>[5x]GAMDIAAQAKLVYHLNKYYNEKCQARKAAIAKTIREVCKVVSDVLKEVEVQEPRFISSLNEMDNRYEGLEVISPTEFEVVLYLNQMGVFNFVDDGSLPGCAVLKLSDGRKRSMSLWVEFITASGYLSARKIRSRFQTLVAQAVDKCSYRDVVKMVADTSEVKLRIRDRYVVQITPAFKCTGIWPRSAAHWPLPHIPWPGPNRVAEVKAEGFNLLSKECHSLAGKQSSAESDA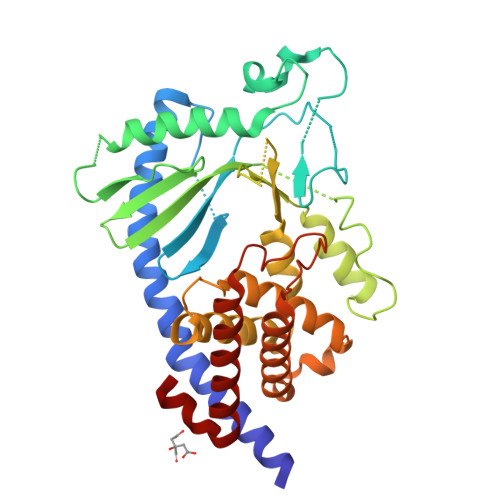WVLQFAEAENRLQMGGCRKKCLSILKTLRDRHLELPGQPLNNYHMKTLVSYECEKHPRESDWDESCLGDRLNGILLQLISCLQCRRCPHYFLPNLDLFQGKPHSALENAAKQTWRLAREILTNPKSLEKL>ATPHINAEMGDFADVVLMPGDPLRAKYIAETFLEDAREVNNVRGMLGFTGTYKGRKISVMGHGMGIPSCSIYTKELITDFGVKKIIRVGSCGAVLPHVKLRDVVIGMGACTDSKVNRIRFKDHDFAAIADFDMVRNAVDAAKALGIDARVGNLFSADLFWSPDGEMFDVMEKYGILGVEMEAAGIYGVAAEFGAKALTICTVSDHIRTHEQT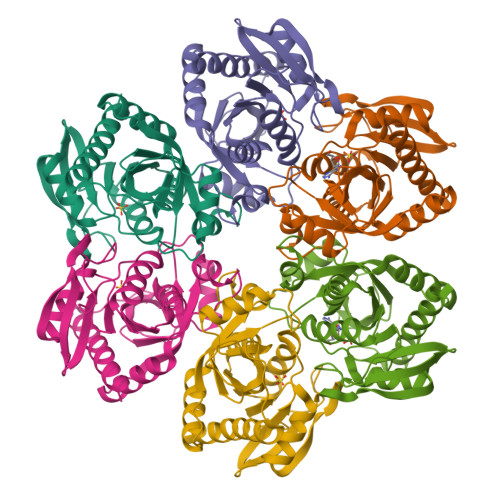TAAERQTTFNDMIKIALESVLLGDK[3x]Flavin-binding fluorescent proteins (FbFPs), engineered from prokaryotic and eukaryotic light, oxygen, voltage (LOV) photoreceptors, are promising fluorescent reporter proteins. Their small size (about 10 kDa for monomeric FbFPs such as the improved LOV (iLOV) protein derived from Arabidopsis thaliana phototropin photoreceptors) and their oxygen-independent fluorescence make them ideal reporters to monitor transport and anaerobic biological processes. In contrast to GFP-like fluorescent reporter proteins, whose absorption and fluorescence maxima can be tuned by exchanging certain chromophore-constituting amino acids, the absorption and fluorescence of FbFPs and other flavoproteins depends on noncovalently bound flavins, whose structure cannot be influenced by mutation. Using spectroscopy, X-ray crystallography, and quantum mechanics molecular mechanics calculations, we provide a firm structural and functional understanding of spectral tuning in FbFPs.

To verify the transferability of the blue-shifting Q489K mutation, identified for the plant FbFP iLOV, we introduced the corresponding Q148K mutation into the recently presented thermostable CagFbFP protein from thermophilic phototrophic bacterium Chloroflexus aggregans. Much like iLOV–Q489K, CagFbFP–Q148K possesses a blue-shifted S0→S1 absorption band with a maximum at around 444 nm (≈3 nm blue-shifted relative to parental CagFbFP) and a blue-shifted fluorescence-emission maximum (≈6 nm blue shift relative to parental CagFbFP; compare the gray dashed line and solid blue line). To verify that the structural changes, which we observed for iLOV–Q489K, are indeed a consequence of the introduced Q489K mutation and are not due to the observed succinimide modification, we obtained the structure of the corresponding CagFbFP–Q148K variant. Altogether, we were able to obtain three types of CagFbFP–Q148K crystals, all using the precipitant solutions with pH of 6.5 (data and refinement statistics are summarized in Table S1). Interestingly, the protein also crystallized using another precipitant solution for which we obtained crystals in two crystal forms. In all of the obtained models, the C terminus of the protein is clearly unlatched, and the side chain of the introduced lysine is facing away from FMN as was found in iLOV–Q489K. Thus, the succinimide modification present in iLOV–Q489K does not influence the backbone and the conformation of the introduced Lys because this modification is absent in all CagFbFP–Q148K structures. Therefore, we conclude that irrespective of the buffer and post-translational modification, the C terminus of the iLOV–Q489K and CagFbFP–Q148K variants is unlatched, the LOV core domain is opened up to allow solvent ingress, and the introduced lysine occupies an extended conformation facing away from the FMN chromophore. The photophysical properties of the CagFbFP variants are relatively straightforward to interpret.

>[2x]MASGMIVTDAGADQPIVFVNRAFSTITGYAPNEVLGRNARFLQGPQTDAATVARLREAIAAARPIQERILNYRKDGQPFWNQLSISPVRDETGNVVAFVGVKTDVTAHHHHHH> GSSSTAATSRDALPNTEASGPTHSKEIPALTAVETGATNPLVPSDTVQTRHVVQHRSRSESSIESFFARGACVTIMTVDNPASTTNKDKLFAVWKITYKDTVQLRRKLEFFTYSRFDMELTFVVTANFTETNNGHALNQVYQIM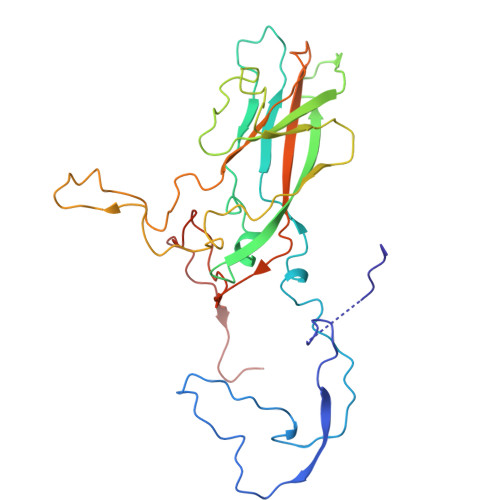YVPPGAPVPEKWDDYTWQTSSNPSIFYTYGTAPARISVPYVGISNAYSHFYDGFSKVPLKDQSAALGDSLYGAASLNDFGILAVRVVNDHNPTKVTSKIRVYLKPKHIRVWCPRPPRAVAYYGPGVDYKDGTLTPLSTKDLTTY>MLSVNEIAAEIVEDMLDYEEELRIESKKLENGAIVVDCGVNVPGSYDAGIMYTQVCMGGLADVDIVVDTINDVPFAFVTEYTDHPAIACLGSQKAGWQIKVDKYFAMGSGPARALALKPKKTYERIEYEDDADV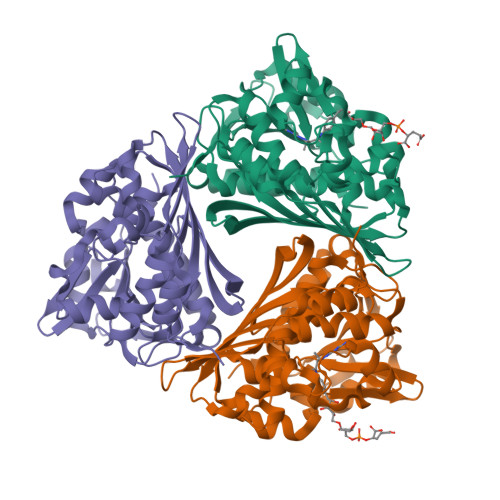AVIALEANQLPDEKVMEFIAKECDVDPENVYALVAPTASIVGSVQISGRIVETAIFKMNEIGYDPKLIVSGAGRCPISPILENDLKAMGSTNDSMMYYGSVFLTVKKYDEILKNVPSCTSRDYGKPFYEIFKAANYDFYKIDPNLFAPAQIAVNDLETGKTYVHGKLNAEVLFQSYQIVLEE[3x]In this study, we used a cyanobacterial BVR from Synechocystis sp. PCC 6803 (Syn BVR)13 as a target for the structural analyses. BVR catalyses the reduction of the C10 double bond (γ-methene bridge) of BV using NAD(P)H to produce BR, a reaction in which the hydride (H−: a proton and two electrons) is donated by NAD(P)H. Syn BVR is composed of 328 residues and shares more than 20% sequence identity with rat and human BVR proteins. Syn BVR consists of two structural domains (N-terminal and C-terminal domains), with the active sites in an obvious cleft between them.

We successfully obtained BV-bound BVR crystals by the co-crystallization screening, and the resulting crystals were a bluish-green colour. The BV-bound crystals belong to a different space group (P21) than those of the apo- and NADP+ soaked forms (P212121), and the asymmetric unit contains four BVR molecules (A to D molecules). Surprisingly, two BV molecules are bound to the catalytic cleft between the two domains, and adopt a stacked configuration along with the tetrapyrrole plane. NADP+ molecules were also bound by all four BVR molecules, although we did not add the NADP+ reagent during the purification and crystallization procedures. The configuration of NADP+ in the ternary complex was identical to that in the NADP+-soaking crystal. One BV (the proximal BV) was bound in close vicinity of the nicotinamide ring, and the other one (the distal BV) was located on the upper stack with the proximal BV. The C10 double bond in the proximal BV, which is to be reduced, faces the nicotinamide C4 carbon (origin of the hydride) of the NADP+; the distance between the C10 carbon of the proximal BV and the C4 carbon of the NADP+ is 2.6 Å, and the angle between the C10 and nicotinamide ring was ∼120°. This configuration of the proximal BV appears suitable to accept the hydride from the nicotinamide ring, and strongly suggests that the hydride is directly transferred to the C10 carbon in the proximal BV. The distal BV is located ∼4 Å above, translated by ∼2.5 Å to the solvent side and rotated ∼45° relative to the proximal BV. Instead, the guanidine group of Arg185 formed hydrogen bonds with the carboxy group of the propionate side chain of the proximal BV (within 2.8 Å in all molecules of the asymmetric unit); thus, the Arg185 must first donate its proton to the propionate side chain of the proximal BV.

>[4x]GSHMSENFAVATPVRVGIVGTGYAAQRRAEVFRGDRRSQLVSFWGNSEANTAKFADTFGVRPQQSWQALINDPEIDLVLIATINQLHGAIAEAALQAGKHVVLEYPLALTYAMGKKLQQLAREKGKLLHVEHIELLGGVHQAIRQNLGKIGEVFYARYSTIMGQNPAPQRWTYHHQQFGFPLVAALSRISRFTDLFGTVQQVDAQCRFWDQPNPEYFRACLATAYLQFNNGLKAEVIYGKGEVFHQNERIFTLHGDRGTLIFVGETGRLIQGQTETEITVGSRRGLFRQDTEAVLDYLTTGKPLYVDLEASLYALEVADLCAQACGYKVEN>SNILEMTKNYYDRSVSPVEYAYFDQSQNMRAINWNKIVDEKDLEVWNRVTQNFWLPENIPVSNDLPSWNELDDDWQQLITRTFTGLTLLDTVQSSIGDVAQIKNSLTEQEQVIYANFAFMVGVHARSYGTIFSTLCTSEQIEEAHEWVVDNEALQARPKALIPFYTADDPLKSKIAAALMPGFLLYGGFYLPFYLSARGKLPNTSDIIRLILRDKVIHNFYSGYKYQLKVAKLSPEKQAEMKQFVFDLLDKMIGLEKTYLHQLYDGFGLADEAIRFSLYNAGKFLQNLGYES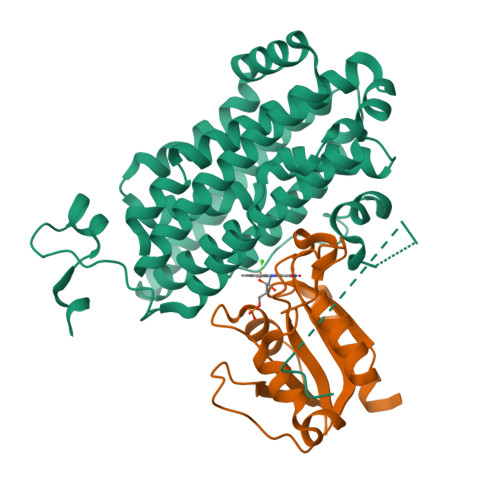PFTKEETRIAPEVFAQLSARADENHDFFSGSGSSYIIGTSEETLDEDWDF[4x];>[4x]SNILEMKELIVYFSTQSNNTHRFVQKLDAESIRIPIDEEERIKVDEDYVLIVPTYSGGKVTDAGQVDAHGAVPKQVIHFLNDPDNRKHCLGVISSGNTNFGDSFAIAGPVISYKLKVPLLYQFELIGTKEDVEEVNRIISETFNADQ> GPGSMSNSRQHQGHFARKRF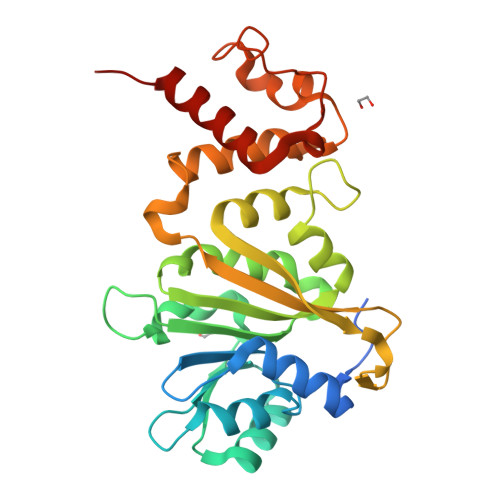GQNFLVDHGVIDAIVAAIRPERGERMVEIGPGLGALTGPVIARLATPGSPLHAVELDRDLIGRLEQRFGELLELHAGDALTFDFGSIARPGDEPSLRIIGNLPYNISSPLLFHLMSFAPVVIDQHFMLQNEVVERMVAEPGTKAFSRLSVMLQYRYVMDKLIDVPPESFQPPPKVDSAIVRMIPHAPHELPAVDPAVLGEVVTAAFSQRRKMLRNTLGGYRDLVDFDALGFDLARRAEDIGVDEYVRVAQAVASARASG methyl 4-{2-[(6-amino-8-oxo-7,8-dihydro-1H-imidazo[4,5-g]quinazolin-2-yl)amino]ethyl}benzoate | C19 H18 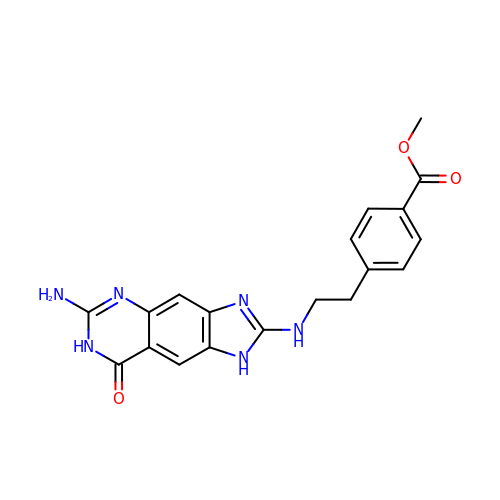N6 O3 | OYIIDOTURROWKC-UHFFFAOYSA-N>HHHHHHSKKPRQKRTATKAYNVTQAFGRRGPEQTQGNFGDQELIRQGTDYKHWPQIAQFAPSASAFFGMSRIGMEVTPSGTWLTYTGAIKLDDK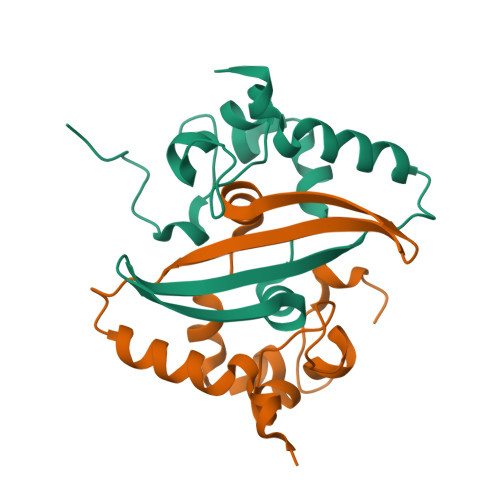DPNFKDQVILLNKHIDAYKTFP[2x]>[4x]GSKEE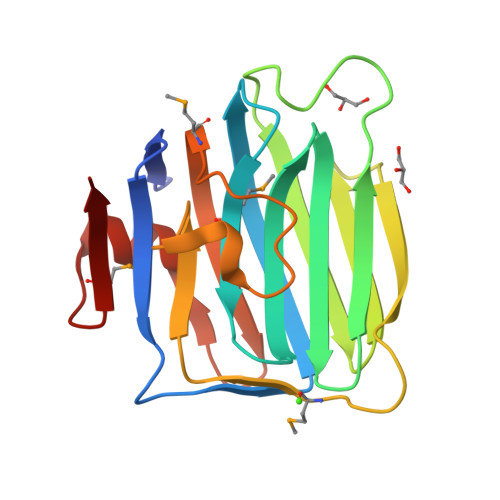YIATFKGSEYFCYDLSQNPIQSSSDEITLSFKTLQRNGLMLHTGKSADYVNLALKNGAVSLVINLGSGAFEALVEPVNGKFNDNAWHDVKVTRNLRQVTISVDGILTTTGYTQEDYTMLGSDDFFYVGGSPSTADLPGSPVSNNFMGCLKEVVYKNNDVRLELSRLAKQGDPKMKIHGV5-(4-chlorophenyl)-~{N}-(3,5-dimethoxyphenyl)furan-2-carboxamide | C19 H16 Cl N O4 | 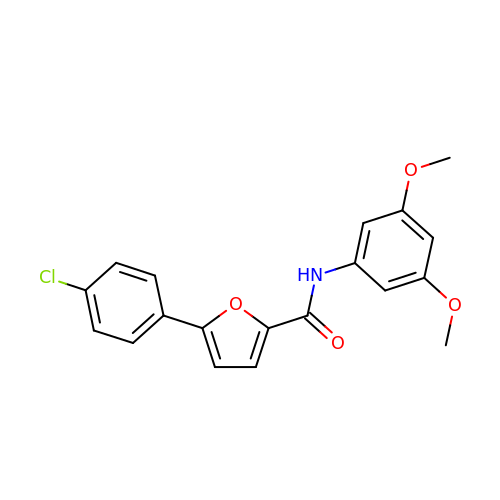VHKBTPQDHDSBSP-UHFFFAOYSA-N By co-opting KBTBD4, a substrate receptor of the CUL3–RING E3 ubiquitin ligase (CRL3) complex, UM171 promotes the degradation of the LSD1–CoREST corepressor complex, thereby limiting haematopoietic stem cell attrition. KBTBD4 contains an N-terminal BTB domain, a central BACK domain and a C-terminal KELCH-repeat propeller domain. As expected, KBTBD4 forms a homodimer through its BTB domain, which is characterized by a domain-swapped two-stranded β-sheet (β1 and β5)34. The predicted CUL3-binding 3-box helices of the KBTBD4 BTB domain are extended by five short helices in the BACK domain, which is connected to the KELCH-repeat domain through a linker sequence. Together, the BTB-BACK modules of the two KBTBD4 protomers give rise to a V-shaped platform, which holds the two KELCH-repeat domains on the same side of the E3 homodimer without physically contacting one another.

For comparison purposes, we also determined the cryo-EM structure of KBTBD4 in its apo form at a resolution of 3.83 Å. In comparison to the LHC-bound structure, the V-shaped platform of the free KBTBD4 dimer adopts a more open conformation. Superposition analysis shows that each protomer in the free KBTBD4 dimer is largely identical to that of the LHC-bound form. However, the BTB N-terminal α1 helix in each protomer is tilted away from the BTB core, thereby flattening the V-shaped scaffold and further separating the two KELCH-repeat domains from one another (from around 9 Å to 30 Å). Thus, UM171-induced LHC binding involves significant conformational changes within the E3, which are accommodated by structural plasticity at the KBTBD4 dimer interface. A comparison between the free and LHC-bound forms of KBTBD4 further reveals an open-to-closed conformational change within the E3 homodimer, underscoring that the actions of glues can benefit from both local and global structural plasticity in E3s. Notably, UM171 binds to a pocket that is present only after KBTBD4-B–HDAC1 contact, suggesting that the surface of E3 scaffolds can be structurally plastic and might contain more binding sites for glue engagement than their apo structures reveal.

>MKGGNADSWQREKLASMESPEEPGASMDENYFVNYTFKDRSHSGRVAQGIMKLCLEEELFADVTISVEGREFQLHRLVLSAQSCFFRSMFTSNLKEAHNRVIVLQDVSESVFQLLVDYIYHGTVKLRAEELQEIYEVSDMYQLTSLFEECSRFLARTVQVGNCLQVMWLADRHSDPELYTAAKHCAKTHLAQLQNTEEFLHLPHRLLTDIISDGVPCSQNPTEAIEAWINFNKEEREAFAESLRTSLKEIGENVHIYLIGKESSRTHSLAVSLHCAEDDSISVSGQNSLCHQITAACKHGGDLYVVGGSIPRRMWKCNNATVDWEWCAPLPRDRLQHTLVSVPGKDAIYSLGGKTLQDTLSNAVIYYRVGDNVWTETTQLEVAVSGAAGANLNGIIYLLGGEENDLDFFTKPSRLIQCFDTETDKCHVKPYVLPFAGRMHAAVHKDLVFIVAEGDSLVCYNPLLDSFTRLCLPEAWSSAPSLWKIASCNGSIYVFRDRYKKGDANTYKLDPATSAVTVTRGIKVLLTNLQFVLA[2x]uridine-5'-diphosphate-3-N-(R-3-hydroxylauroyl)-N-acetyl-D-glucosamine 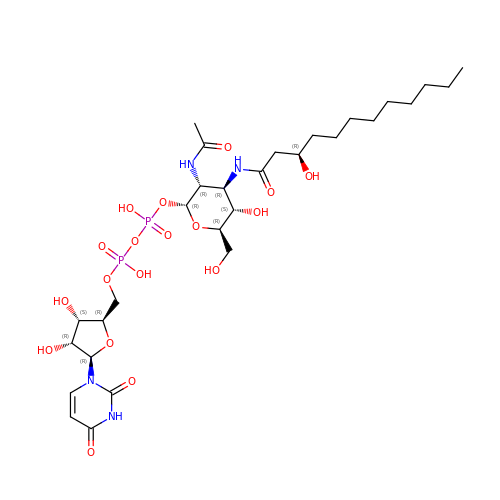| C29 H50 N4 O18 P2 | AGYVEKOUTSGPCD-SSVOXRMNSA-N>[2x]ARQREIEMNRQQRFFRIPFIRPADQYKDPQSK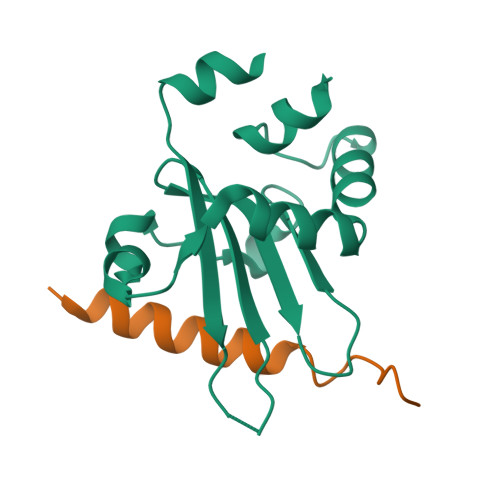KKGWWYAHFDGPWIARQMELHPDKPPILLVAGKDDMEMCELNLEETGLTRKRGAEILPRQFEEIWERCGGIQYLQNAIESRQARPTYATAMLQSLLK;>GVTSEGKFDKFLEERAKAADRLPNLSS[2x]>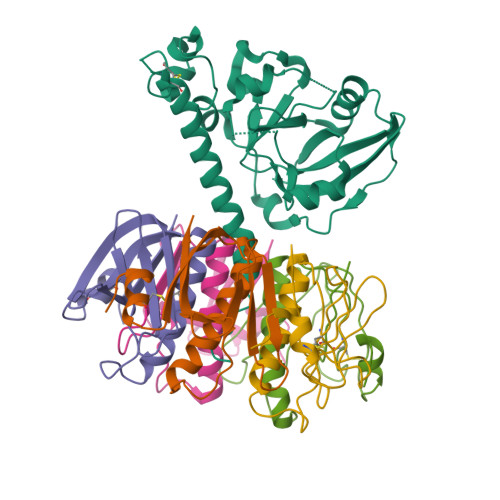 NDDKLYRADSRPPDEIKQSGGLMPRGQSESFDRGTQMNINLYDHARGTQTGFVRHDDGYVSTSISLRSAHLVGQTILSGHSTYYIYVIATAPNMFNVNDVLGAYSPHPDEQEVSALGGIPYSQIYGWYRVHFGVLDEQLHRNRGYRDRYYSNLDIAPAADGYGLAGFPPEHRAWREEPWIHHAPPGCGNAPRSSMSNTCDEKTQSLGVKFLDEYQSKVKRQIFSGYQSDIDTHNRIKDEL;>[5x]TPQNITDLCAEYHNTQIHTLNDKIFSYTESLAGKREMAIITFKNGATFQVEVPGSQHIDSQKKAIERMKDTLRIAYLTEAKVEKLCVWNNKTPHAIAAISMAN N-[(E)-3-[(2R,3S,4S)-3,4-dihydroxyoxolan-2-yl]prop-2-enyl]-2,3-dihydroxy-5-nitro-benzamide | C14 H16 N2 O8 | 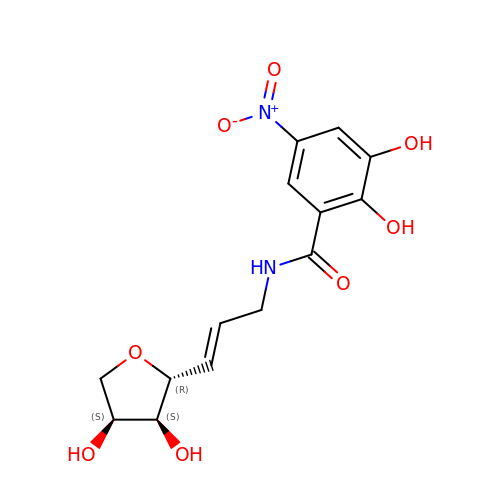VDHNUEGZSFACAM-CNBGNIIQSA-N>MEQKLISEEDLNSAVDHHHHHHRIPGLINSSLKFVVSSLDIIAAQAGRNKQLAELAEKALAAIKENDQQLPDPEVVFAPLQLATKSGTIPLTTTALDCIGKLISYSYFSAPSSSATQDGTEQTPLIERAIDTICDCFQGETTLVEIQLQIVKSLLAAVLNDKIIVHGAGLLKAVRQVYNIFLLSRSTANQQVAQGTLTQMVGTVFERVKTRLHMKEARANLGRLKASRSSLAVDRSDDQDSQAGKVDGEDATVETVSDATPSESVDKAGGGKLTLKDLEHRKSFDDSHMGDGPTMVSQVKPMKKASRSVSEQSLQESPQDETPESLDAEDEAYIRDAYLVFRSFCNLSTKILPPDQLYDLRGQPMRSKLISLHLIHTLLNNHITVFTSPLCTIRNTKNNEPTNFLQAIKYYLCLSITRNGASSVDRVFDICCEIFWLMLKYMRSSFKNEIEVFLNEIYLALLARRNAPLSQKLTFVGILKRLCEDPRALVELYLNYDCNQNVDNIFQTIVEDLSRFATASVPITPTQEQQYEESRSKSATAGEWQIKSVLPPPLSVALIATNHEADTELPKEYVMKRTALDSLVETLRSLVHWSQPGRPELNGASGDVQRRTSSDDLGDSIDPSMSETASRMEVPIAPATPVIDDDPDQLEKEKARKTAMTNAIKVFNFKPKHGIKLLIKEGFIPSDKPEDIARFLLREERLDKAQIGEYLGEGDQKNVDIMHAFVDMMDFSKKRFVDALREFLQAFRLPGEAQKIDRFMLKFAHRYVTGNPNAFANADTPYVLAYSVIMLNTDLHSSKVVKRMSKAEFIKNNRGINDNADLPDEYLIGIYDDIASNEIVLKSEREAAAAAGTLPAQSTGLAGLGQAFSNVGRDLQREAYVQQSEEISLRSEQLFRDLYRSQRKSATKGGVKFISATSFKHVGPMFDATWMSFFSTLSSLVQKTHNLDVNKLCLEGMKLATKIACLFDLSTPREAFISMLKNTANLNNPREMQAKNVEALKVLLDLAQTEGNYLKESWKDVLLCISQLDRLQLISGGVDESAVPDVSRARFVPPPRTETGESRKSTSSARRTRPRAHTGPQGVSLEIALESRSDEVIKSVDRIFTNTANLSRDAIIHFARALTEVSWDEIKVSGSNDSPRTYSLQKIVEISYYNMTRVRFEWSHIWDVLGEHFNRVGCHANTAIVFFALDSLRQLSMRFMEIEELAGFKFQKDFLKPFEHVMSNSSNVTVKDMVLRCLIQMIQARGENIRSGWRTMFGVFTVAAREPYESIVNLAYENVTQVYKTRFGVVISQGAFTDLIVCLTEFSKNMRFQKKSLQAMETLKSVIPTMLKTPECPLSQHKPTATTASGSESHSKKAAVQQTRTSVEEGFWFPVLFAFHDVLMTGEDLEVRSNALNYFFETLLRYGGDFPPEFWDILWRQQLYPIFMVLRSRPEMTNALNHEELSVWLSTTMIQALRNMITLFTHYFDALEYMLDRFLELLA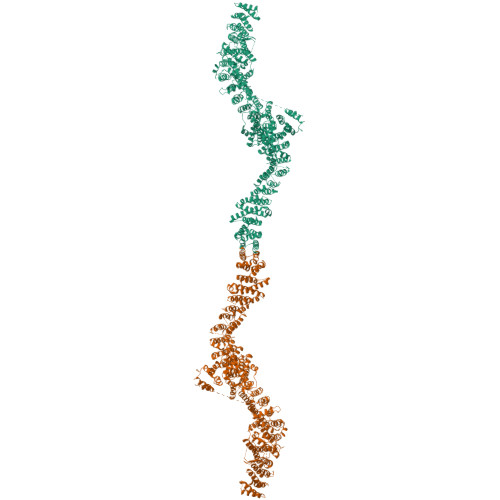LCICQENDTIARIGSNCLQQLILQNVTKFTAEHWAKIVGAFCELFERTTAYQLFSATTINSTASLSPPPSGLELGGPLSPTSATAPVDGKSLKINGVETNGQTPGAEPANGDADGNGTAAAAADASAPAATPQPQQGPAQQLEEFKPNNPLQQQPVVVTAARRRFFNRIISRCVLQLLMIETVNELFSNDAVYAQIPSAELLRLMALLKKSFLFAKRFNADKDLRMRLWREGFMKQPPNLLKQESGSAATYVAILFRMFGDTAPDRRGSRADVEAALVPLCRDIIRGYTALDDESQHRNIVAWRPVVVDVLEGYAAFPRDAFAAHIRSFYPLVVELLGKDLGQDLRAALLLVLRRVGEVGLGIEGMGSGGAAAAAAAGAAAASSGQGNGNGAAAAAADSERRSSVLSVPSGPRHTPSMDSLNDDPSRQVMGKAEQKLISEEDLNSAVDHHHHHH[2x]>MEKPTPLINSSMLGQYVGQTVRIVGKVHKVTGNTLLMQTSDLGNVEIAMTPDSDVSSSTFVEVTGKVSDAGSSFQANQIREFTTVDCGHDVDLTLVENVVQISAAFPNLFSDST[2x];>GKKAGNNTLRPVTIRQILNAEQPHPDAEFILDGAELGQLTFVAVVRNISRNATNVAYSVEDGTGQIEVRQWLDSSSDDSSKASEIRNNVYVRVLGTLKSFQNRRSISSGHMRPVIDYNEVMFHRLEAVHAHLQVTR[2x];>MPIYPIEGLSPYQNRWTIKARVTSKSDIRHWSNQRGEGKLFSVNLLDDSGEIKATGFNDAVDRFYPLLQENHVYLISKARVNIAKKQFSNLQNEYEITFENSTEIEECTDATDVPEVKYEFVRINELESVEANQQCDVIGILDSYGELSEIVSKASQRPVQKRELTLVDQGNRSVKLTLWGKTAETFPTNAGVDEKPVLAFKGVKVGDFGGRSLSMFSSSTMLINPDITESHVLRGWYDNDGAHAQFQPYTNGGVGGGAMGGGGAGANMAERRTIVQVKDENLGMSEKPDYFNVRATVVYIKQENLYYTACASEGCNKKVNLDHENNWRCEKCDRSYATPEYRYILSTNVA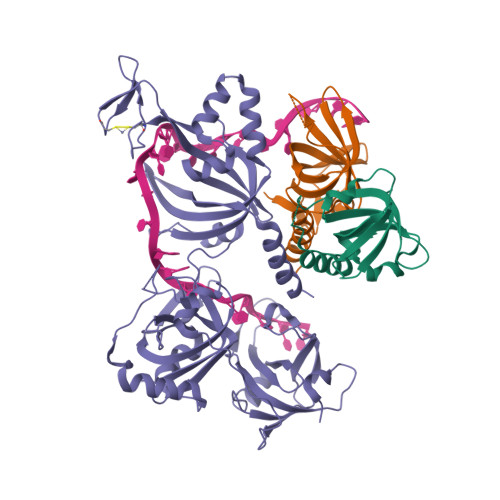DATGQMWLSGFNEDATQLIGMSAGELHKLREESESEFSAALHRAANRMYMFNCRAKMDTFNDTARVRYTISRAAPVDFAKAGMELVDAIRAYM[2x]>MKKIKPHGPLPSQTQLAYLGDELAAFIHFGPNTFYDQEWGTGQEDPERFNPSQLDAREWVRVLKETGFKKLILVVKHHDGFVLYPTAHTDYSVKVSPWRRGKGDLLLEVSQAATEFDMDMGVYLSPWDAHSPLYHVDREADYNAYYLAQLKEILSNPNYGNAGKFAEVWMNGARGEGAQKVNYEFEKWFETIRDLQGDCLIFSTEGTSIRWIGNQRGYAGDPLWQKVNPDKLGTEAELNYLQHGDPSGTIFSIGEADVSIRPGWFYHEDQDPKSLEELVEIYFHSVGRGTPLLLNIPPNQAGLFDAKDIERLYEFATYRNELYKEDLALGAEVSGPALSADFACRHLTDGLETSSWASDADLPIQLELDLGSPKTFDVIE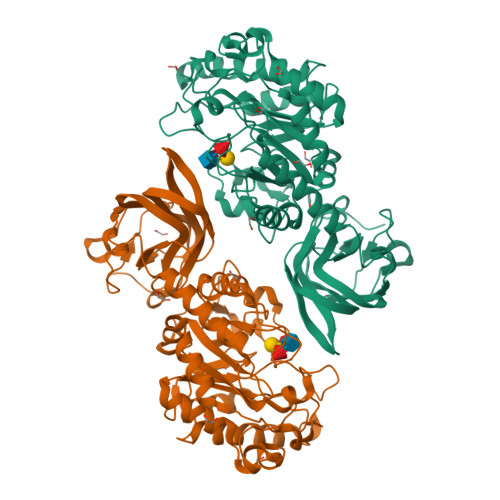LREDLKLGQRIAAFHVQVEVDGVWQEFGSGHTVGYKRLLRGAVVEAQKIRVVITESQALPLLTKISLYKTP[2x]> MSASAELEPDVKGRILDAAADAFMARGFANTTIDDIADEVGATKGLIYYHFRSKFDIFLAVYEDGMRRVRERVEPHSTAPGTGHQRLEAMSIAHLENLMTELGYHHVVHQ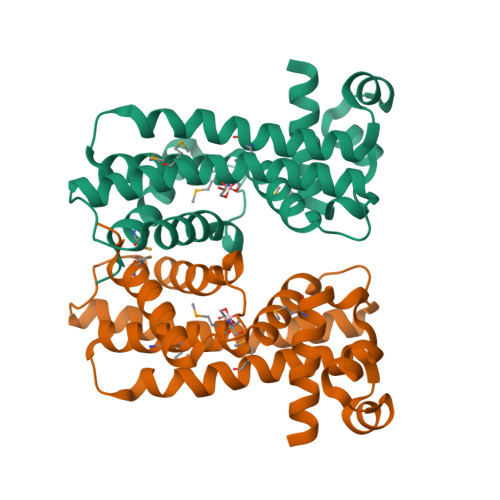GVRHQDSTALKVRQRDALTALNELRRDYERMFRRVIAEGIADGSLRRVDEALATRTLLSNLNAVDVWYRKIEGQTGEEIRELASQVVDMLIGGLAD Cypoviruses, members of the family Reoviridae, subfamily Spinareovirus, possess a single capsid layer with turrets and are commonly embedded in crystalline occlusion bodies called polyhedra, which are formed in the cell cytoplasm and mainly composed of a single virus-encoded protein, polyhedrin. To ensure the delivery of virus particles to the target intestinal cells, allowing the transmission of packages of infectious virus between hosts by oral-faecal routes, polyhedra are disrupted only when they are exposed to the very alkaline pH environment found in insect midguts. The fold of all the polyhedrins is highly similar – a β-barrel core sitting on a base domain, surrounded by a common array of five helices (H1–H5). The strongest intermolecular interactions define a trimer composed of a cluster of three β-barrels sandwiched by helices top and bottom.

CPV20 has elongated V1 and V5 but unlike CPV4 they do not interact. CPV4, 5 and 20 lack both ATP and GTP, whilst the other cypovirus types have varying combinations, in all cases the V1, V3, V4, V2c or V5 regions of the protein adopt alternate polypeptide conformations. In CPV20 the V4 loop is similarly shortened whilst V1, V2c, and V5 infiltrate the region. NTP binding in this area is only observed in CPV1 and CPV20. The pyridine in CPV20 is not well ordered, but can be identified as UTP based on the limited space and the hydrogen bonding environment provided by residue 101 main chain nitrogen and the side chain nitrogen of H79, whilst the triphosphates are supported by two lysines, two histidines and an arginine. The pyridines stabilise the dodecamer, although in CPV1 the CTPs also interact with each other, whilst the UTPs in CPV20 are more deeply buried in the trimer interface. In CPV1, 14, 15, 17, 18 and 20 solvent molecules can move between these two voids, whereas in CPV4, 5 and 19 they are blocked by tyrosine residues. CPV1, CPV19 and CPV20 were resistant such that only a small portion was dissolved in an hour while the other six cypovirus types plus the two deletion mutants dissolved dramatically. In fact the three CPVs (CPV1, 19 and 20) most resistant to alkali buffers all display more extensive interactions between the 3-fold symmetry-related subunits of the trimeric building block – strengthened by either pyridine binding (CPV1 and CPV20) or numerous protein–protein hydrogen bonds.

> XSNQPFNQPNVLQERQHLVNRQLVQGPNVQDAIKRVAIIFIYKNGSYRLIDYNAPEFINGYFNWRDMLYMDKPAHSNRHKEFENQIRRPDHGDSHHPELFEYPVAIMISANGNICWENVRVEVENEDCLNHEDWRRARAWGPRCYKGSQMMKCSALGRFLYIPLRCQNESLKFKFPSRMSGGDNRYSSHSIGQVIQNNIIIRNNPLYLDNEGDLIDYMQAKNLCYIDSAAVVDCNGLAGDSEC> GNKYIQQTKPLTLERTINLYPLTNYTFGTKEPLYEKDSSVAARFQRMREEFDKIGMRRTVEGVLIVHEHRLPHVLLLQLGTTFFKLPGGELNPGEDEVEGLKRLMTEILGR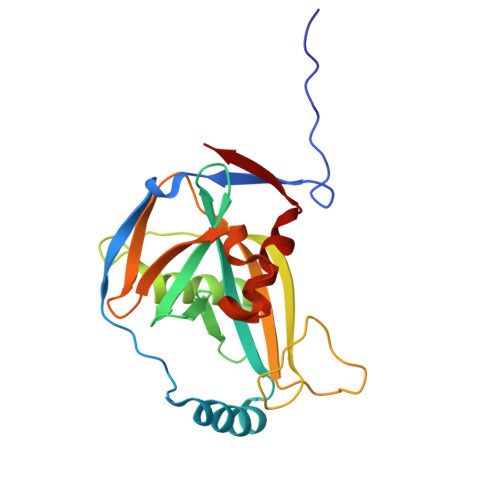QDGVLQDWVIDDCIGNWWRPNFEPPQYPYIPAHITKPKEHKKLFLVQLQEKALFAVPKNYKLVAAPLFELYDNAPGYGPIISSLPQLLSRFNFIYN>MIFPGATVRVTNVDDTYYRFEGLVQRVSDGKAAVLF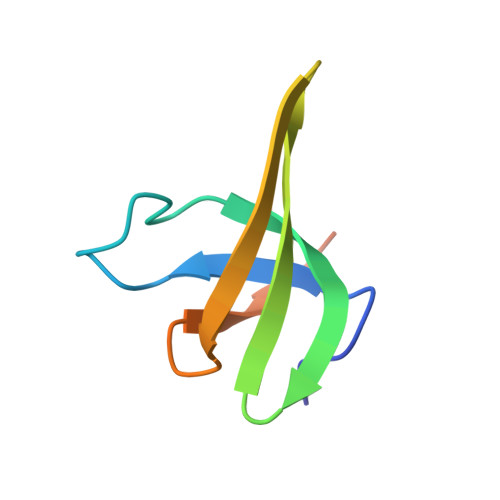ENGNWDKLVTFRLSELEAVKPILEHHHHHH[2x]>[2x]EELPAPVKAIEKQGITIIKTFDAPGGMKGYLGKYQDMGVTIYLTPDGKHAISGYMYNEKGENLSNTLIEKEIYAPAGREMWQRMEQSHWLLDG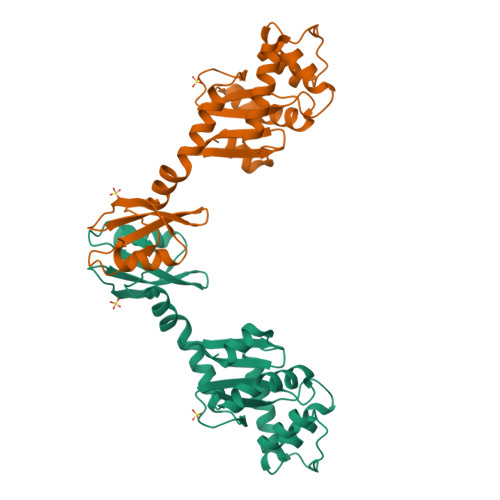KKDAPVIVYVFADPFCPYCKQFWQQARPWVDSGKVQLRTLLVGVIKPESPATAAAILASKDPAKTWQQYEASGGKLKLNVPANVSTEQMKVLSDNEKLMDDLGANVTPAIYYMSKENTLQQAMGLPDQKTLNIIMGNKHHHHHH>SVAILQKRDHEGFGFVLRGAKAETPIEEFTPTPAFPALQYLESVDVEGVAWKAGLRTGDFLIEVNGV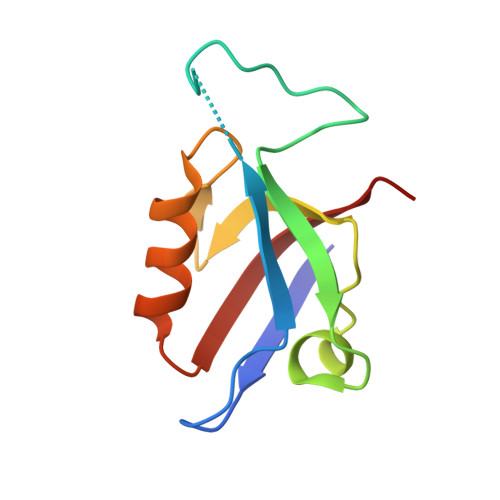NVVKVGHKQVVGLIRQGGNRLVMKVVSVT[2x]>MAADAPAASQQSKPSESDKSESSMSSHAPVVFTLRTGIAEGRMVYIGVGGDIDRQVNPKLVVHEGETVQINLINGEGAQHDAVIDQYAARSAIVSGKNASSTFSFIASKVGQFDYYCSLPGHRQAGMQGVLQVVPGNRAEMPSTAADITRDPADLPGPIGARQAKTVRIDLETVELKGQLDDKTTYTYWTFNGKVPGPFLRVRVGDTVELHLKNAKDSLMIHSVDFHGATGPGGAAAYTQTDPGAETVVTFKALVPGIFVYHCATPSVPNHITNGMYGLLLVEPEGGLPQVDREFYVMQGEIYTVKPFGTSGEQEMDYEKLISEKPEYFLFNGSVGALTRTHPLYANVGETVRIFFGVGGPNFTSSFHVIGEIFDHVYALGSVTSPPLTGVQTVSVPPGGATI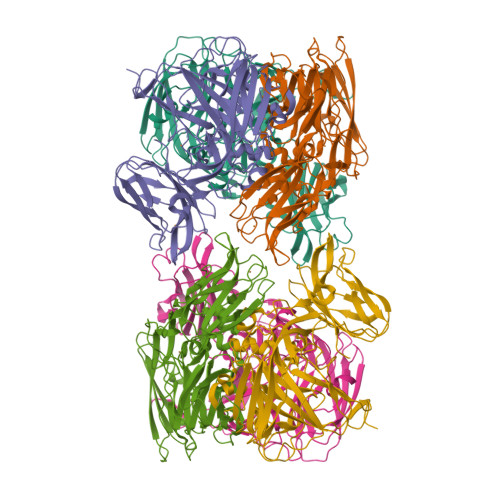VDFKLDRGGRYVLVDHALSRLDHGLVGFLNVDGPKNDAIMHEGPPKQENLYFQ[3x]>[2x]GNSATSADEQPHIGNYRLLKTIGKGNFAKVKLARHILTGKEVAVKIIDKTQLNSSSLQKLFREVRIMKVLNHPNIVKLFEVIETEKTLYLVMEYASGGEVFDYLVAHGRMKEKEARAKFRQIVSAVQYCHQKFIVHRDLKAENLLLDADMNIKIADFGFSNEFTFGNKLDTFCGSPPYAAPELFQGKKYDGPEVDVWSLGVILYTLVSGSLPFDGQNLK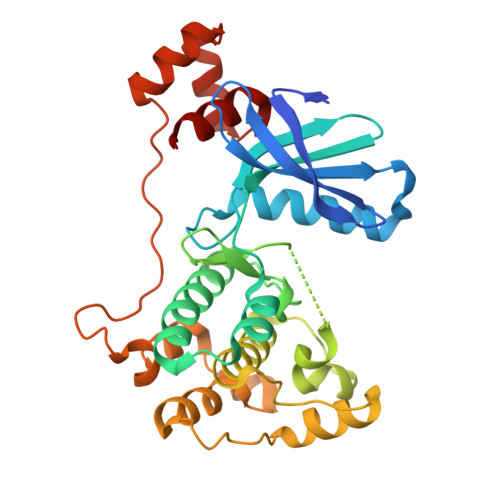ELRERVLRGKYRIPFYMSTDCENLLKKFLILNPSKRGTLEQIMKDRWMNVGHEDDELKPYVAPLPDYKDPRRTELMVSMGYTREEIQDSLVGQRYNEVMATYLLLGYK>GAMATLQERVAAHFAESIRAKQEAEKILVEPTVQAAELMLQCLMNDGKILACGNGGSAADAQHFAAEMTGRFEKERMELAAVALTTDTSALTAIGNDYGFDHVFSKQVRALGRAGDVLVGISTSGNSANVIEAVKAAHERDMHVIALTGRDGGKIAAMLKDTDVLLNVPHPRTARIQENHIL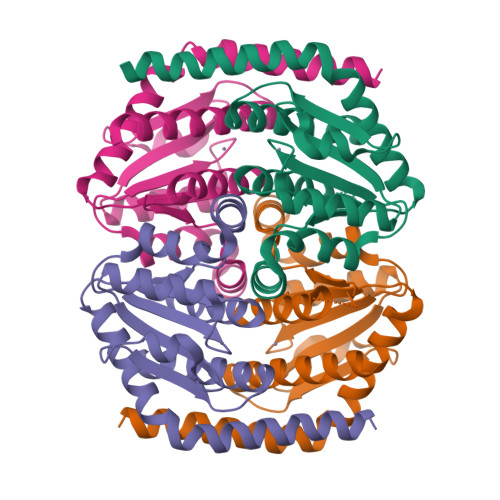LIHAMCDCIDSVLLEGMKLAAA[4x]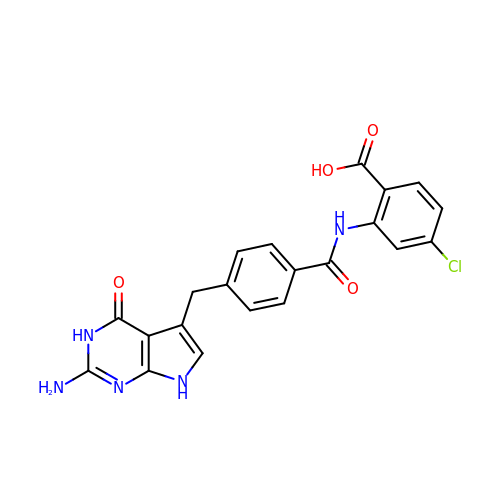2-({4-[(2-amino-4-oxo-4,7-dihydro-3H-pyrrolo[2,3-d]pyrimidin-5-yl)methyl]benzene-1-carbonyl}amino)-4-chlorobenzoic acid | C21 H16 Cl N5 O4 | OBHYLCXTIVOOGV-UHFFFAOYSA-N> MESSDVELDFQRSVQAVLRELNTPNPALQSNQGMWRWSLHKKVERNPGKSSILVRILLRELEKAESEDGRRVIIPLLLTLMSVLTKATGIPEDLYHRAYTFCTRLLTLPAPYSTVALDCAIRLKTETAVPGTLYQRTVIAEQNLISELYPYQERVFLFVDPELVSASVCSALLLEIQAAQEQQTPEACMRHVVSHALQAALGEACHTGALNRKLQASSRRVLEYYFHAVVAAIEQVASEDSPSRLGHLEKMEEIYCSLLGPATTRRHCVGDLLQDRLPSIPLPSPYITFHLWTDQEQLWKELVLFLRPRSQLRLSADLDALDLQGFRLDRDLARVSTDSGIERDLPLGSDELPDPSSSEMERAALQRKGGIKKRVWPPDFFMPGSWDGPPGLHRRTGRPSGDGELLPGVSRVHTARVLVLGDDRMLGRLAQAYYRLRKRETKKFCLTPRLSLQLYYIPVLAPQVTGQDPEASRKPELGELASFLGRVDPWYESTVNTLCPAILKLAEMPPYLDTSRTVDPFILDVITYYVRMGTQPIYFQLYKVKIFTSLSHDPTEDIFLTELKVKIQDSKSPKEGSSPRRRGAAEGTGAELSMCYQKA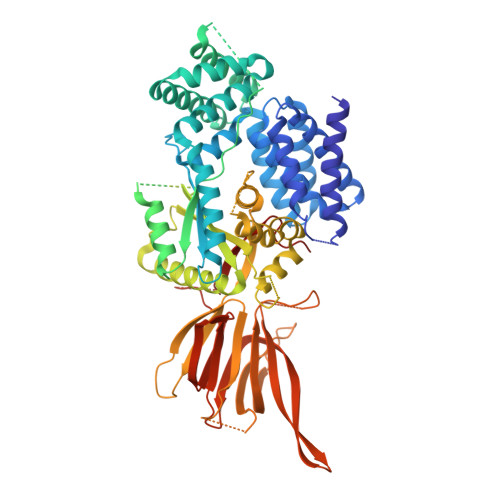LLSHRPREVTVSLRATGLVLKAIPAGDTEVSGFFHCTSPNAASATDCSCLHVSVTEVVKSSNLAGRSFTTSTNTFRTSSIQVQSQDQRLLTLWLDKDGRRTFRDVVRFEVSPCPEPCSRTQKSKTSALNSHGQETEKNMAKPNSLLMPINTFSGIIQ> GPGSEFELPLPEGWEEARDFDGKVYYIDHRNRTTSWIDPRDRYTKPLTFADCISDELPLGWEEAYDPQVGDYFIDHNTKTTQIEDP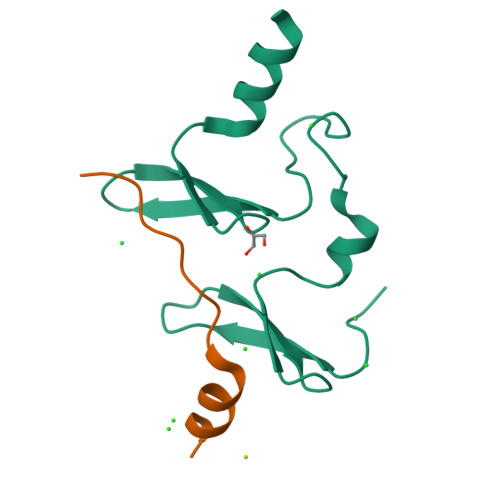RVQWRREQEHMLKDYLVVAQEALSAQKEIYQVKQQRLELAQQEYQQLH;> GPGSSHRHSAIIVPSYRPTPDYETVMRQMKRG5-methylfuran-2-carboxylic 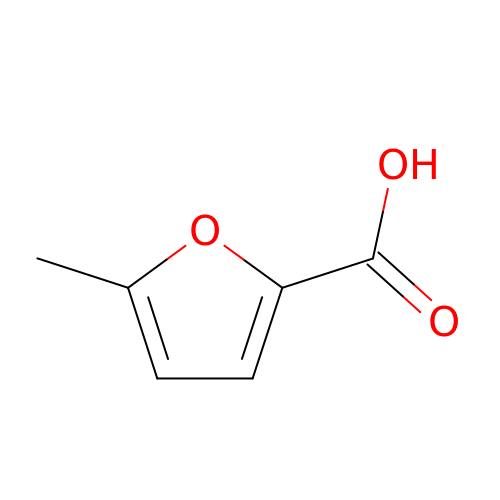acid | C6 H6 O3 | OVOCLWJUABOAPL-UHFFFAOYSA-N>[4x]MSDQQQPPVYKIALGIEYDGSKYYGWQRQNEVRSVQEKLEKALSQVANEPITVFCAGRTDAGVHGTGQVVHFETTALRKDAAWTLGVNANLPGDIAVRWVKTVPDDFHARFSATARRYRYIIYNHRLRPAVLSKGVTHFYEPLDAERMHRAAQCLLGENDFTSFRAVQCQSRTPWRNVMHINVTRHGPYVVVDIKANAFVHHMVRNIVGSLMEVGAHNQPESWIAELLAAKDRTLA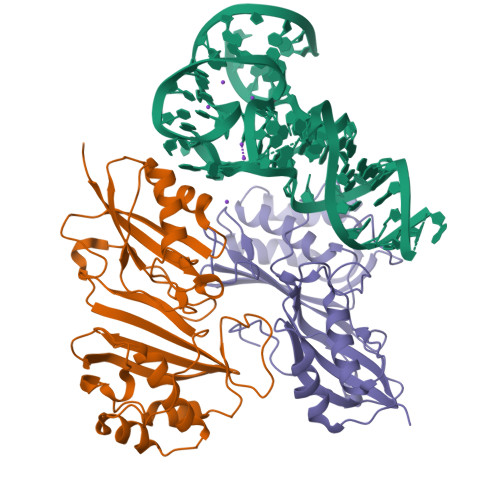AATAKAEGLYLVAVDYPDRYDLPKPPMGPLFLAD(2R)-N-{4-[(3-bromophenyl)sulfonyl]-2-chlorophenyl}-3,3,3-trifluoro-2-hydroxy-2-methylpropanamide 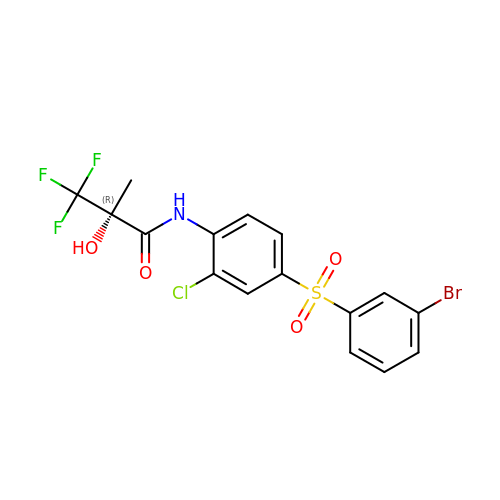| C16 H12 Br Cl F3 N O4 S | NPCYFKFOPWAEFV-OAHLLOKOSA-N Among the SLC4 transporters, Na+-dependent members function as either symporters or exchangers that mediate their specific physiologic roles in different cell types by thermodynamically coupling the transport of Na+ to base (HCO3− or CO32−) with or without simultaneous Cl− transport. To further improve our general understanding of these transporters, we investigated the structural and functional properties of human NBCe1, a Na+-coupled SLC4 symporter, using cryo electron microscopy (cryoEM) and functional mutagenesis studies. The transporter is a member of the anion exchanger family belonging to the APC superfamily, the second largest secondary carrier superfamily. The 3.9 Å structure of NBCe1 provides a common framework for the Na+-coupled SLC4 transporters that underlies their functional properties.

NBCe1 was solubilized in 1% Triton X-100, purified and exchanged into PMAL-C8 amphipol resulting in well-dispersed particles. By combining ~185,000 best particles, we obtained a cryoEM reconstruction at near-atomic (3.9 Å) resolution. The reconstruction contains two NBCe1 monomers with identical structures and its side view resembles the iconic double-headed eagle with its body, wing, head and foot corresponding to the gate domain, the core domain, extracellular loop 3 (EL3) domain and the cytoplasmic region of each monomer, respectively. Each NBCe1 monomer consists of 14 TMs (divided into two structurally related inverted repeats: TMs 1–7 and TMs 8–14), with four amphipathic helices (H1-4), a short (single turn) cytoplasmic helix (H5), and the loops connecting all these helices. Densities for the cytoplasmic N-terminus (Met1-Gly400), the distal portion of EL3 (Cys583-Leu637), EL4 (Ser713-Trp734), intracellular loop 5 (IL5; Glu814-Lys825) and the cytoplasmic C-terminus (Asp966-Cys1035) were less well-resolved due to the dynamic nature of these regions and were not modeled. Our atomic model of the NBCe1 monomer is arranged into gate and core domains. The region corresponding to the middle of the transporter within each monomer formed by short TM3 and TM10 and the antiparallel β-strands preceding these TMs has been proposed to contribute to substrate coordination in other transporters. This region of NBCe1 is accessible from the extracellular side as predicted by HOLE2 representing an outward-open conformation. The pathway contains an electropositive opening from the extracellular side with an external diameter >12 Å and the most constricted region (~2 Å diameter) formed by TM3, TM10, and the antiparallel β-strands in the middle of each NBCe1 monomer. In addition to Thr485, our structure and mutagenesis data suggests that Ser483 (the β-strand preceding TM3), Ser484 (the β-strand preceding TM3), Asp754 (TM8), Thr758 (TM8), and Thr801 (TM10) are also involved in ion coordination.

>[2x]MSTENVEGKPSNLGERGRARSSTFLRVVQPMFNHSIFTSAVSPAAERIRFILGEEDDSPAPPQLFTELDELLAVDGQEMEWKETARWIKFEEKVEQGGERWSKPHVATLSLHSLFELRTCMEKGSIMLDREASSLPQLVEMIVDHQIETGLLKPELKDKVTYTLLRKHRHQTKKSNLRSLADIGKTVSSASRMFTNPDNGSPAMTHRNLTSSSLNDISDKPEKDQLKNKFMKKLPRDAEASNVLVGEVDFLDTPFIAFVRLQQAVMLGALTEVPVPTRFLFILLGPKGKAKSYHEIGRAIATLMSDEVFHDIAYKAKDRHDLIAGIDEFLDEVIVLPPGEWDPAIRIEPPKSLPSSDKRKNMYSGGENVQMNGDTPHDGGHGGGGHGDCEELQRTGRFCGGLIKDIKRKAPFFASDFYDALNIQALSAILFIYLATVTNAITFGGLLGDATDNMQGVLESFLGTAVSGAIFCLFAGQPLTILSSTGPVLVFERLLFNFSKDNNFDYLEFRLWIGLWSAFLCLILVATDASFLVQYFTRFTEEGFSSLISFIFIYDAFKKMIKLADYYPINSNFKVGYNTLFSCTCVPPDPANISISNDTTLAPEYLPTMSSTDMYHNTTFDWAFLSKKECSKYGGNLVGNNCNFVPDITLMSFILFLGTYTSSMALKKFKTSPYFPTTARKLISDFAIILSILIFCVIDALVGVDTPKLIVPSEFKPTSPNRGWFVPPFGENPWWVCLAAAIPALLVTILIFMDQQITAVIVNRKEHKLKKGAGYHLDLFWVAILMVICSLMALPWYVAATVISIAHIDSLKMETETSAPGEQPKFLGVREQRVTGTLVFILTGLSVFMAPILKFIPMPVLYGVFLYMGVASLNGVQFMDRLKLLLMPLKHQPDFIYLRHVPLRRVHLFTFLQVLCLALLWILKSTVAAIIFPVMILALVAVRKGMDYLFSQHDLSFLDDVIPEKDKKKKEDEKKKKKKKGSLDSDNDDSDCPYSEKVPSIKIPMDIMEQQPFLSDSKPSDRERSPTFLERHTSC>LSISDASATEPGSGGIAPGFLRTSGNQILDSQGKPVQLTGVNWFGAQSSNGVPDGLWTRNYKDMIDQMAGQGFNTIRIPYASALLHTNAAPSGINYNANPDLQGLTRMQVLDKIIDYAGQAGMRVILDHHRSTEGAGTSENGLWYDSQYTEDAWVSDWQTLATRYKNNPTVIGFDLHNEPYNGTWGGGGANDWARAAERAGNAALAINPNLLIIVEGVGSYKGDNYWWGGQLQGVKDRPIQLNVANRVVYSPHDYP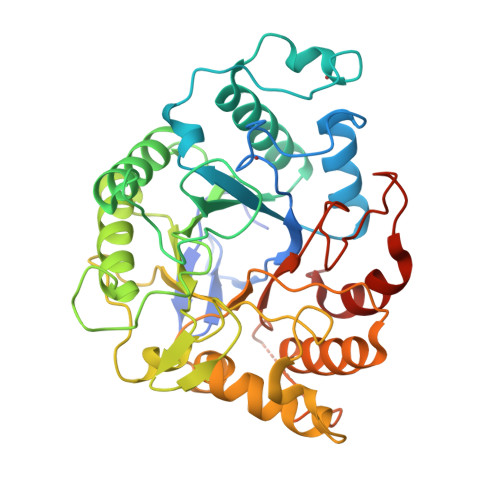NSVWQQPWFQGDNFGAGLPAKFRSEWGYIYEQNIAPIYIGEFGTKLIDPKDAVWLEALTSYLSGDFDNNGTIDIPAGTEDMSWTFWSWNPNSGDTGGILADDWRTINQNKMVYLKPIQYTGGNGT[8x]2-(4-{[2-(2,6-difluorophenyl)-5-oxo-5H-pyrrolo[3,4-d]pyrimidin-4-yl]amino}phenyl)-N-ethylacetamide | 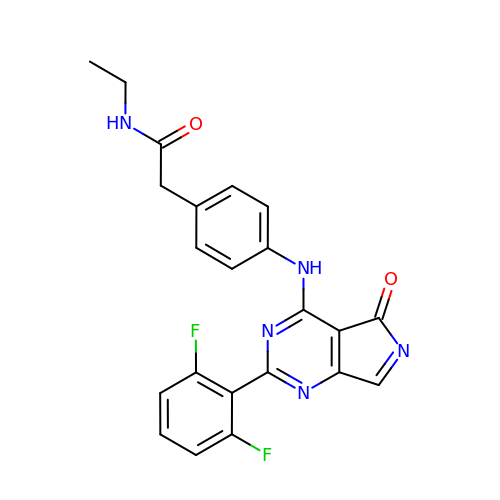C22 H17 F2 N5 O2 | JPMGFORVJWNXAQ-UHFFFAOYSA-N>[44x]MDMLFAK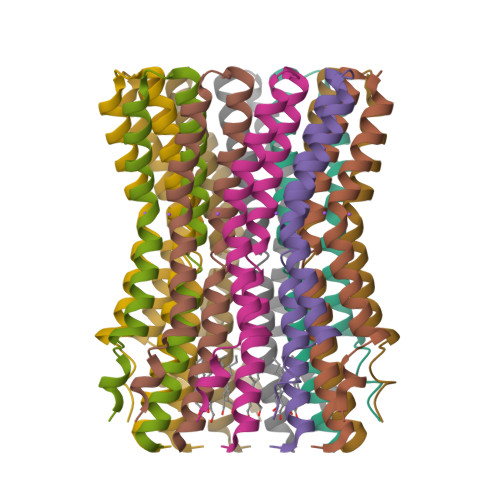TVVLAASAVGAGTAMIAGIGPGVGQGYAAGKAVESVARQPEAKGDIISTMVLGQAVAESTGIYSLVIALILLYANPFVGLLG N-[(3S)-1-({6-chloro-3-[1-(4-chlorobenzyl)-4-phenyl-1H-imidazol-5-yl]-1H-indol-2-yl}carbonyl)pyrrolidin-3-yl]-N,N',N'-trimethylpropane-1,3-diamine 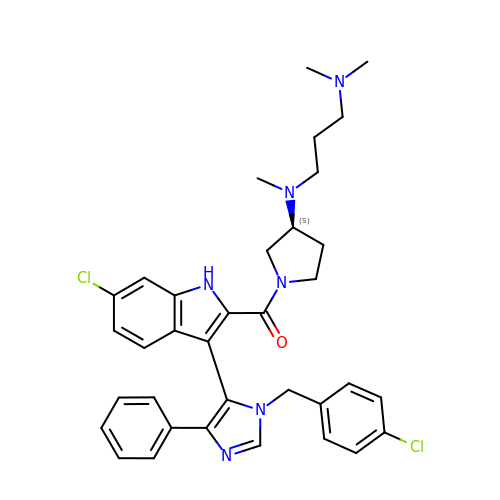| C35 H38 Cl2 N6 O | LWWQYOWAPGRPRH-NDEPHWFRSA-N> GMAEGNTLISVDYEIFGKVQGVFFRKHTQAEGKKLGLVGWVQNTDRGTVQGQLQGPISKVRHMQEWLETRGSPKSHIDKANFNNEKLIEELDYSDFQIVA

As the sole target of neutralizing antibodies, the virion surface protein Env encodes a glycan shield to restrict the antibody access to antigenically conserved sites. Small protein mimics of the CONEs are designed by epitope transplantation and used as immunogens to focus the antibody response. Here we focus our protein design efforts on four CONEs, including the structural elements of β sheet 12/13/22 (CONE 1), α2 helix (CONE 2), loop C (CONE 4), and loop E (CONE 5).

The CONE 4 (loop C) residues were grafted onto the C-terminal loop region of an α/β mixed protein. A characteristic array of three glutamic acids flanked by hydrophobic residues defines the conformation of CONE 4 loop in Env. Our design largely recapitulates the conformations of two charged side chains (E88 and E89). The hydrophobic residue L86 also adopts a similar conformation to L265 of Env. Comparison with the Env trimer protein revealed a high degree of mimicry: within the epitope region, the Cα RMSDs between the designed proteins and Env were 0.42 Å (C2S5) and 0.34 Å (C4S3), respectively, suggesting that our CONE mimetics accurately display the Env residues. The electron density maps revealed that the side chains of the grafted residues were well positioned relative to the computational model. As a control experiment, we also immunized five rabbits with a synthetic peptide of the CONE 4 sequence (LAEEEI). None of these rabbits could induce antisera of significant titers, in contrast to the C4S3-immunized rabbits, indicating that for a linear epitope, constraining it in the right conformation with suitable protein scaffolds is favorable for the generation of functional antibodies. The CONE 4 (loop C) and CONE 5 (loop E) immunogens did induce HIV-specific antibodies as assessed by ELISA and western blot assay. The purified IgG fractions of anti-CONE 4 and anti-CONE 5 rabbit sera bound to the deglycosylated form of gp120 but not the glycosylated protein. Most of the animals immunized with C4S3 also generated antibodies that bound to the deglycosylated SOSIP Env protein, whereas no such antibodies were detected in animals immunized with C5S3.>[4x]MTELAQLQASAEQAAALLKAMSHPKRLLILCMLSGSPGTSAGE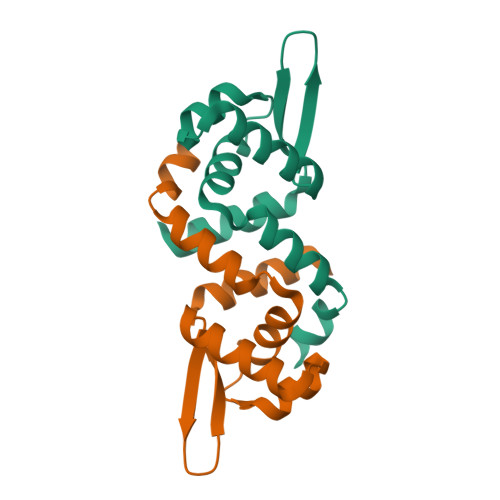LTRITGLSASATSQHLARMRDEGLIDSQRDAQRILYSIKNEAVNAIIATLKNVYCP> GPLG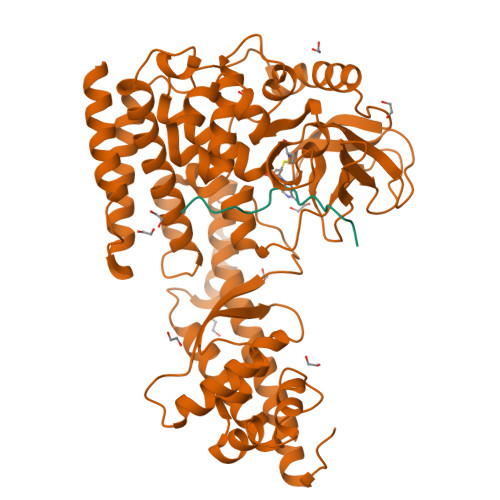SMGKKSRVKTQKSGTGATATVSPKEILNLTSELLQKCSSPAPGPGKEWEEYVQIRTLVEKIRKKQKGLSVTFDGKREDYFPDLMKWASENGASVEGFEMVNFKEEGFGLRATRDIKAEELFLWVPRKLLMTVESAKNSVLGPLYSQDRILQAMGNIALAFHLLCERASPNSFWQPYIQTLPSEYDTPLYFEEDEVRYLQSTQAIHDVFSQYKNTARQYAYFYKVIQTHPHANKLPLKDSFTYEDYRWAVSSVMTRQNQIPTEDGSRVTLALIPLWDMCNHTNGLITTGYNLEDDRCECVALQDFRAGEQIYIFYGTRSNAEFVIHSGFFFDNNSHDRVKIKLGVSKSDRLYAMKAEVLARAGIPTSSVFALHFTEPPISAQLLAFLRVFCMTEEELKEHLLGDSAIDRIFTLGNSEFPVSWDNEVKLWTFLEDRASLLLKTYKTTIEEDKSVLKNHDLSVRAKMAIKLRLGEKEILEKAVKSAAVNREYYRQQMEEKAPLPKYEESNLGLLESSVGDSRLPLVLRNLEEEAGVQDALNIREAISKAKATENGLVNGENSIPNGTRSENESLNQESKRAVEDAKGSSSDSTAGVKE;> TLKYPIEHGIVTNWD> MLEAKFEEASLFKRIIDGFKDCVQLVNFQCKEDGIIAQAVDDSRVLLVSL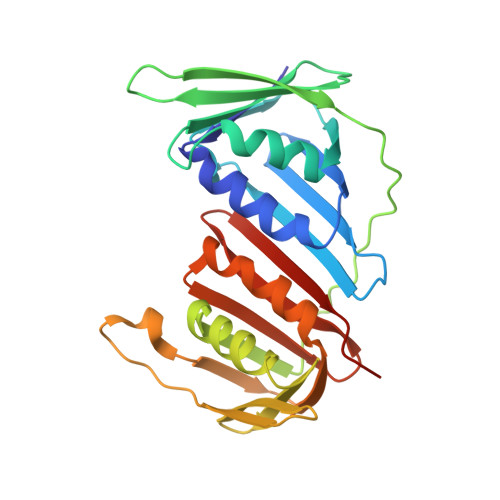EIGVEAFQEYRCDHPVTLGMDLTSLSKILRCGNNTDTLTLIADNTPDSIILLFEDTKKDRIAEYSLKLMDIDADFLKIEELQYDSTLSLPSSEFSKIVRDLSQLSDSINIMITKETIKFVADGDIGSSSVIIKPFVDMEHPETSIKLEMDQPVDLTFGAKYLLDIIKGSSLSDRVGIRLSSEAPALFQFDLKSGFLQFFLAPKFNDEE(2S)-2,3-dihydroxypropyl (9Z)-octadec-9-enoate 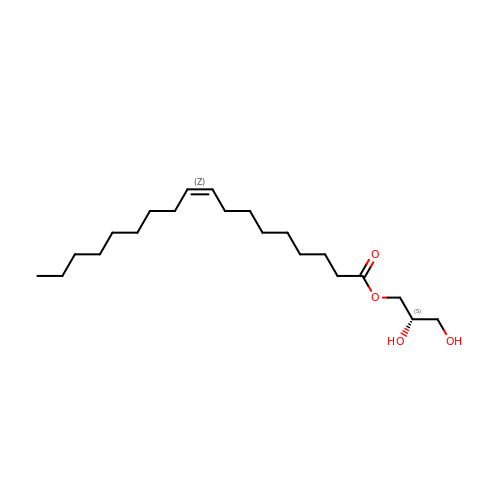| C21 H40 O4 | RZRNAYUHWVFMIP-QJRAZLAKSA-N> MRYRLAWLLHPALPSTFRSVLGARLPPPERLCGFQKKTYSKMNNPAIKRIGNHITKSPEDKREYRGLELANGIKVLLISDPTTDKSSAALDVHIGSLSDPPNIAGLSHFLQHMLFLGTKKYPKENEYSQFLSEHAGSSNAFTSGEHTNYYFDVSHEHLEGALDRFAQFFLSPLFDESAKDREVNAVDSEHEKNVMNDAWRLFQLEKATGN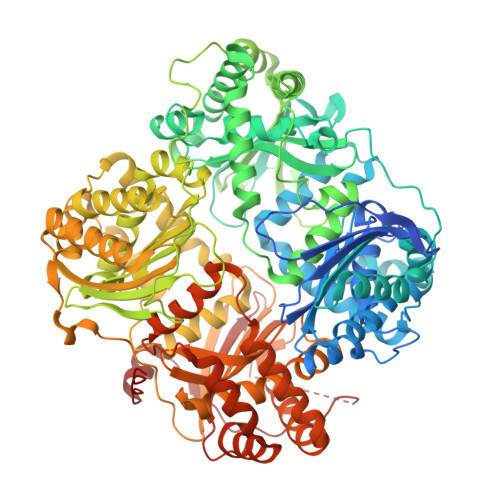PKHPFSKFGTGNKYTLETRPNQEGIDVRQELLKFHSAYYSSNLMAVVVLGRESLDDLTNLVVKLFSEVENKNVPLPEFPEHPFQEEHLKQLYKIVPIKDIRNLYVTFPIPDLQKYYKSNPGHYLGHLIGHEGPGSLLSELKSKGWVNTLVGGQKEGARGFMFFIINVDLTEEGLLHVEDIILHMFQYIQKLRAEGPQEWVFQELKDLNAVAFRFKDKERPRGYTSKIAGILHYYPLEEVLTAEYLLEEFRPDLIEMVLDKLRPENVRVAIVSKSFEGKTDRTEEWYGTQYKQEAIPDEVIKKWQNADLNGKFKLPTKNEFIPTNFEILPLEKEATPYPALIKDTAMSKLWFKQDDKFFLPKANLNFEFFSPFAYVDPLHSNMAYLYLELLKDSLNEYAYAAELAGLSYDLQNTIYGMYLSVKGYNDKQPILLKKIIEKMATFEIDEKRFEIIKEAYMRSLNNFRAEQPHQHAMYYLRLLMTEVAWTKDELKEALDDVTLPRLKAFIPQLLSRLHIEALLHGNITKQAALGIMQMVEDTLIEHAHTKPLLPSQLVRYREVQLPDRGWFVYQQRNEVHNNSGIEIYYQTDMQSTSENMFLELFAQIISEPAFNTLRTKEQLGYIVFSGPRRANGIQGLRFIIQSEKPPHYLESRVEAFLITMEKSIEDMTEEAFQKHIQALAIRRLDKPKKLSAESAKYWGEIISQQYNFDRDNTEVAYLKTLTKEDIIKFYKEMLAVDAPRRHKVSVHVLAREMDSNPVVGEFPAQNDINLSQAPALPQPEVIQNMTEFKRGLPLFPLVKPHINFMAAKL In the present study, we perform a detailed biochemical characterization of the BAI1/ELMO2 interaction, and find that an evolutionarily conserved fragment located in the intracellular region of BAI1 specifically binds to the RBD-ARR-ELMO (RAE) tandem of ELMO2. To elucidate the assembly of BAI1/ELMO2 complex, we solve the crystal structures of the RAE tandem of ELMO2 and its complex with BAI1 at 2.5-Å and 1.7-Å resolutions, respectively. The RBD, ARR and ELMO domains of ELMO2 bind tightly and form a structural and functional supramodule, creating a highly conserved elongated concave groove capable of specifically binding to the BAI1 fragment. Each member consists of the Ras-binding domain (RBD), the armadillo repeats domain (ARR), the engulfment and motility (ELMO) domain, the pleckstrin homology (PH) domain and the C-terminal proline rich region (PRR).

To delineate how then the BAI1-EBD is recognized by this ELMO2-RAE supramodule, we solved the crystal structure of ELMO2-RAE in complex with a synthetic BAI1-EBD peptide at 1.7-Å resolution using the molecular replacement method. Each asymmetric unit contains one BAI1/ELMO2 complex with 1:1 stoichiometry, consistent with our biochemical data. There is no significant conformational change in the RAE tandem of ELMO2 upon binding to BAI1-EBD. Except the N-terminal 4 residues and the C-terminal 7 residues, the electron densities of the rest of the BAI1-EBD (i.e., aa 1471-1495) are clearly defined in the complex. The BAI1-EBD peptide, composed of two short α-helices, occupies the elongated concave groove formed by the ARR and ELMO domains. The complex assembly is mainly mediated by two parts of interactions: (1) the C-terminus of BAI1-EBD forms extensive polar interactions with ELMO2-RAE. For example, R1489BAI1 forms a salt bridge with E198ELMO2; H1485BAI1 forms hydrogen bonds with E281ELMO2 and E429ELMO2, and the sidechain of H284ELMO2 forms hydrogen bonds with the mainchain of I1483BAI1 and sidechain of N432ELMO2; (2) the N-terminus of BAI1-EBD mainly forms hydrophobic interactions with ELMO2-RAE. The hydrophobic core is formed by Tyr1475, Leu1478, Phe1480, Ile1483, Met1484 from BAI1-EBD and Leu202, Leu244, Val288, Leu292, Pro427 from ELMO2-RAE. Particularly, S1473BAI1, R1474BAI1, E248ELMO2, R251ELMO2, E298ELMO2 form a hydrogen bond network. Notably, the binding site of BAI1 on ELMO2 is far away from the RhoG-binding site, suggesting that RhoG and BAI1 would not compete with each other when binding to ELMO2-RAE.

> GPGSMPPPSDIVKVAIEWPGANAQLLEIDQKRPLASIIKEVCDGWSLPNPEYYTLRYADGPQLYITEQTRSDIKNGTILQLAISPSRAARQLMERTQSSNMETRLDAMKELAKLSADVTFATEFINMDGIIVLTRLVESGTKLLSHYSEMLAFTLTAFLELMDHGIVSWDMVSITFIKQIAGYVSQPMVDVSILQRSLAILESMVLNSQSLYQKIAEEITVGQLISHLQVSNQEIQTYAIALINALFLKAPEDKRQDMANAFAQKHLRSIILNHVIRGNRPIKTEMAHQLYVLQVLTFNLLEERMMTKMDPNDQAQRDIIFELRRIAFDAESDPSNAPGSGTEKRKAMYTKDYKMLGFTNHINPAMDFTQTPPGMLALDNMLYLAKVHQDTYIRIVLENSSREDKHECPFGRSAIELTKMLCEILQVGELPNEGRNDYHPMFFTHDRAFEELFGICIQLLNKTWKEMRATAEDFNKVMQVVREQITRALPSKPNSLDQFKSKLRSLSYSEILRLRQSERMSQDD;> RKSRYAELDFEKIMHTRKRHQDMFQ> MSMLKREDWYDLTRTTNWTPKYVTENELFPEEMSGARGISMEAWEKYDEPYKITYPEYVSIQREKDSGAYSIKAALERDGFVDRADPGWVSTMQLHFGAIALEEYAASTAEARMARFAKAPGNRNMATFGMMDENRHGQIQLYFPYANVKRSRKWDWAHKAIHTNEEAAIAARSFFDDMMMTRDSVAVSIMLTFAFETGFS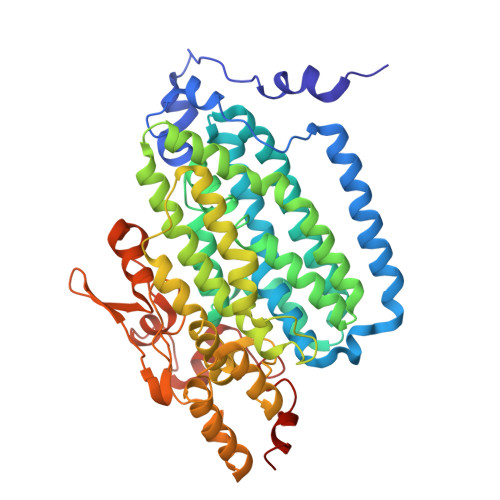NMQFLGLAADAAEAGDHTFASLISSIQTDESRHAQQGGPSLKILVENGKKDEAQQMVDVAIWRSWKLFSVLTGPIMDYYTPLESRNQSFKEFMLEWIVAQFERQLLDLGLDKPWYWDQFMQDLDETHHGMHLGVWYWRPTVWWDPAAGVSPEEREWLEEKYPGWNDTWGQCWDVITDNLVNGKPELTVPETLPTICNMCNLPIAHTPGNKWNVKDYQLEYEGRLYHFGSEADRWCFQIDPERYKNHTNLVDRFLKGEIQPADLAGALMYMSLEPGVMGDDAHDYEWVKAYQKKTNAA>AVSSSRGGITVLTHSELSAEIGVTDSIVVSSELVMPYTVGTWLRGVAANWSKYSWLSVRYTYIPSCPSSTAGSIHMGFQYDMADTVPVSVNQLSNLRGYVSGQVKSGSAGLCFINGTRCSDTSTAISTTLDVSKLGKK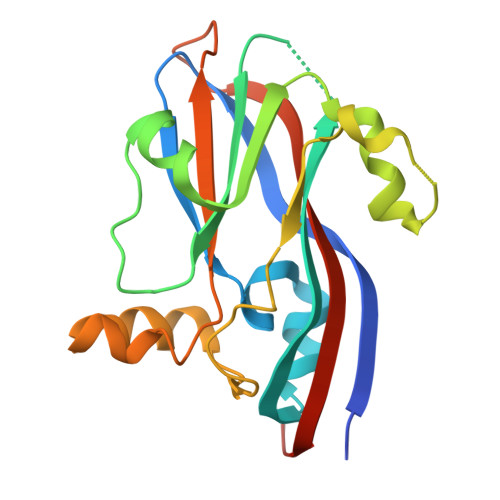WYPYKTSADYATAVGVDVNIATPLVPARLVIALLDGSSSTAVAAGRIYCTYTIQMIEPTASALNN[2x]> GAMAPHFKEELRNLNVRYQSNATLVCKVTGHPKPIVKWYRQGKEIIADGLK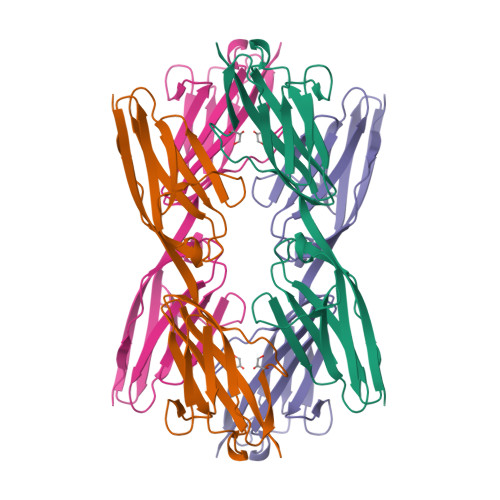YRIQEFKGGYHQLIIASVTDDDATVYQVRATNQGGSVSGTASLEVEVPAKIHLPKTLEGMGAVHALRGEVVSIKIPFSGKPDPVITWQKGQDLIDNNGHYQVIVTRSFTSLVFPNGVERKDAGFYVVCAKNRFGIDQKTVELDVAD6-ethylpyridin-2-amine | 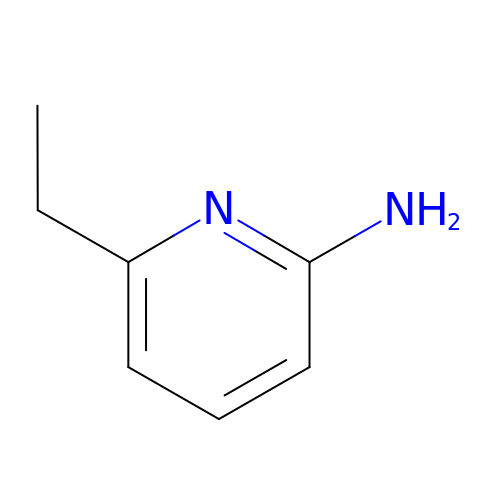C7 H10 N2 | JXKAUUVMXZIJNZ-UHFFFAOYSA-N>MDSGTEEYELNGGLPPGTPGSPDASPARWGWRHGPINVNHYASKKSAAESMLDIALLMANASQLKAVVEQGPSFAFYVPLVVLISISLVLQIGVGVLLIFLVKYDLNNPAKHAKLDFLNNLATGLVFIIVVVNIFITAFGVQKPL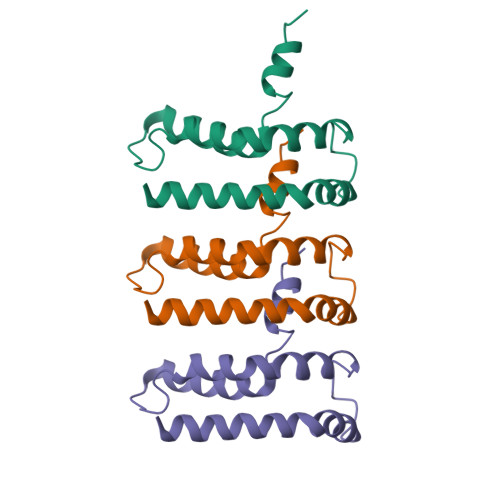MDMAPQQ[3x]>[2x]MPIPNNPGAGENAFDPVFVKDDDGYDLDSFMIPAHYKKYLTKVLVPN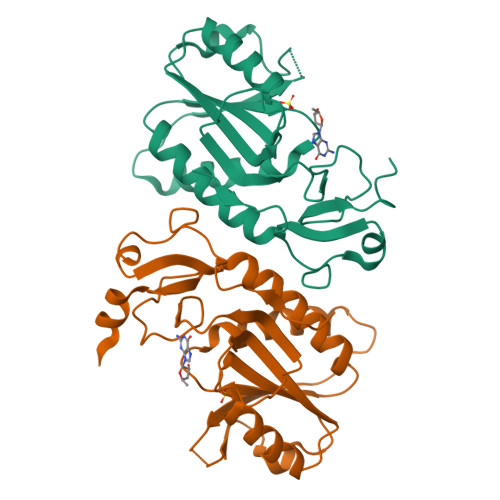GVIKNRIEKLARDVMKEMGGHHIVALCVLKGGYKFFADLLDYIKALNRNSDRSIPMTVDFIRLKSYCNDQSTGDIKVIGGDDLSTLTGKNVLIVEDIIDTGKTMQTLLSLVRQYNPKMVKVACLFIKRTPLWNGFKADFVGFSIPDHFVVGYSLDYNEIFRDLDHCCLVNDEGKKKYKATSL>[4x]MKRSLRKMWRPGEKKEPQGVVYEDVPDDTEDFKESLKVVFEGSAYGLQNFNKQKKLKTCDDMDTFFLHYAAAEGQIELMEKITRDSSLEVLHEMDDYGNTPLHCAVEKNQIESVKFLLSRGANPNLRNFNMMAPLHIAVQGMNNEVMKVLLEHRTIDVNLEGENGNTAVIIACTTNNSEALQILLNKGAKPCKSNKWGCFPIHQAAFSGSKECMEIILRFGEEHGYSRQLHINFMNNGKATPLHLAVQNGDLEMIKMCLDNGAQIDPVEKGRCTAIHFAATQGATEIVKLMISSYSGSVDIVNTTDGCHETMLHRASLFDHHELADYLISVGADINKIDSEGRSPLILATASASWNIVNLLLSKGAQVDIKDNFGRNFLHLTVQQPYGLKNLRPEFMQMQQIKELVMDEDNDGCTPLHYACRQGGPGSVNNLLGFNVSIHSKSKDKKSPLHFAASYGRINTCQRLLQDISDTRLLNE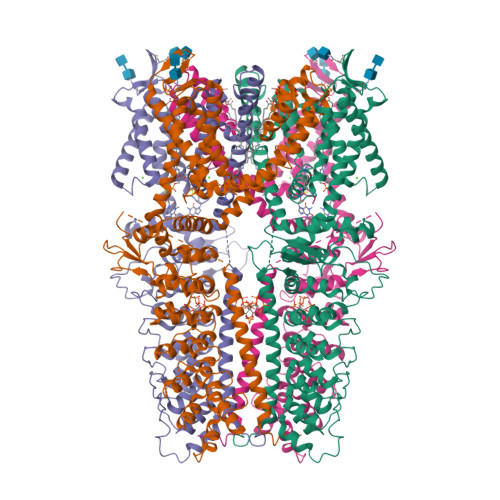GDLHGMTPLHLAAKNGHDKVVQLLLKKGALFLSDHNGWTALHHASMGGYTQTMKVILDTNLKCTDRLDEDGNTALHFAAREGHAKAVALLLSHNADIVLNKQQASFLHLALHNKRKEVVLTIIRSKRWDECLKIFSHNSPGNKCPITEMIEYLPECMKVLLDFCMLHSTEDKSCRDYYIEYNFKYLQCPLEFTKKTPTQDVIYEPLTALNAMVQNNRIELLNHPVCKEYLLMKWLAYGFRAHMMNLGSYCLGLIPMTILVVNIKPGMAFNSTGIINETSDHSEILDTTNSYLIKTCMILVFLSSIFGYCKEAGQIFQQKRNYFMDISNVLEWIIYTTGIIFVLPLFVEIPAHLQWQCGAIAVYFYWMNFLLYLQRFENCGIFIVMLEVILKTLLRSTVVFIFLLLAFGLSFYILLNLQDPFSSPLLSIIQTFSMMLGDINYRESFLEPYLRNELAHPVLSFAQLVSFTIFVPIVLMNLLIGLAVGDIAEVQKHASLKRIAMQVELHTSLEKKLPLWFLRKVDQKSTIVYPNKPRSGGMLFHIFCFLFCTGEIRQEIPNADKSLEMEILKQKYRLKDLTFLLEKQHELIKLIIQKMEIISETEDDDSHCSFQDRFKKEQMEQRNSRWNTVLRAVKAKTHHLEPAENLYFQ>MRGSHHHHHHGLVPRGSMIRTMLQGKLHRVKVTHADLHYEGSCAIDQDFLDAAGILENEAIDIWNVTNGKRFSVYAIAAERGSRIISVNGAAAHCASVGDIVIIASFVTMPDEEARTWRPNVAYFEGDNEMKRTAKAIPVQVA[2x]

Aspartate α-decarboxylase is a pyruvoyl-dependent decarboxylase required for the production of β-alanine in the bacterial pantothenate (vitamin B5) biosynthesis pathway. The enzyme catalyses the decarboxyl­ation of aspartate via the formation of an imine link between the α-amino group of the amino acid and an N-terminal pyruvoyl group. The pyruvoyl group is formed via the intramolecular rearrangement of a serine residue to generate a backbone ester intermediate which is cleaved to generate an N-terminal pyruvoyl group. The activated protein therefore consists of two chains, the N-terminal β-­chain and the C-terminal α-chain, which includes the N-terminal pyruvoyl group formed from Ser25.

To further investigate the role of Thr57 in activation, we determined the three-dimensional structure of the T57V mutant. The T57V mutant ADC crystallized in space group P6122 under similar conditions to those used in previous studies and was subsequently cryoprotected using sodium malonate. Three bands were observed for all site-directed mutants other than T57V. Initial analysis suggested that Thr57 is required for activation, as the T57V mutant cannot be catalytically activated in E. coli at 37°C. Ramjee et al. observed an increased rate of autocatalytic activation of purified ADC at higher temperatures. In this region, the structures of both protomers are similar to each other but in both cases are distinct from the structure observed for the WT zymogen. The hydrogen-bond interaction observed between Ser25 and the β-amide of Asn72 in the WT zymogen is lost owing to these changes in the torsional angles of the chain. The presence of bound malonate in the crystal structure leads to displacement of the unprocessed chain. This means that it is not possible to determine whether the observed conformation in the zymogen is owing to the hydrogen bond between Thr57 and the carbonyl of Gly24, but it may be that the very lack of this hydrogen bond is critical in allowing malonate to bind. A structural analysis of the zymogen reveals that substantial backbone rearrangement occurs as a result of the adventitious binding of a molecule of malonate in the region of the unformed active site; however, there is no evidence for ester formation in the protein, suggesting that Thr57 is required for the formation of the ester intermediate.>MSAPTPLAEASQIPTIPALSPLTAKQSKGNFFSSNPISSFVVDTYKQLHSHRQSLELVNPGTVENLNKEVSRDVFLSQYFFTGLRADLNKAFSMNPAFQTSHTFSIGSQALPKYAFSALFANDNLFAQGNIDNDLSVSGRLNYGWDKKNISKVNLQISDGQPTMCQLEQDYQASDFSVNVKTLNPSFSEKGEFTGVAVASFLQSVTPQLALGLETLYSRTDGSAPGDAGVSYLTRYVSKKQDWIFSGQLQANGALIASLWRKVAQNVEAGIETTLQAGMVPITDPLMGTPIGIQPTVEGSTTIGAKYEYRQSVYRGTLDSNGKVACFLERKVLPTLSVLFCGEIDHFKNDTKIGCGLQFETAGNQELLMLQQGLDADGNPLQALPQL[2x];>MVELTEIKDDVVQLDEPQFSRNQAIVEEKASATNNDVVDDEDDSDSDFEDEFDENETLLDRIVALKDIVPPGKRQTISNFFGFTSSFVRNAFTKSGNLAWTLTTTALLLGVPLSLSILAEQQLIEMEKTFDLQSDANNILAQGEKDAAATANRTLQVDGSPGHHHHHHHHHH[2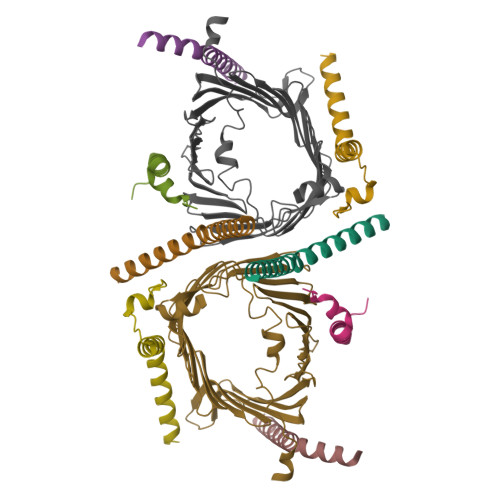x];>MFGLPQQEVSEEEKRAHQEQTEKTLKQAAYVAAFLWVSPMIWHLVKKQWK[2x];>[2x]MDGMFAMPGAAAGAASPQQPKSRFQAFKESPLYTIALNGAFFVAGVAFIQSPLMDMLAPQL;>[2x]MSFLPSFILSDESKERISKILTLTHNVAHYGWIPFVLYLGWAHTSNRPNFLNLLSPLPSV>[2x]GRKKRVEISAP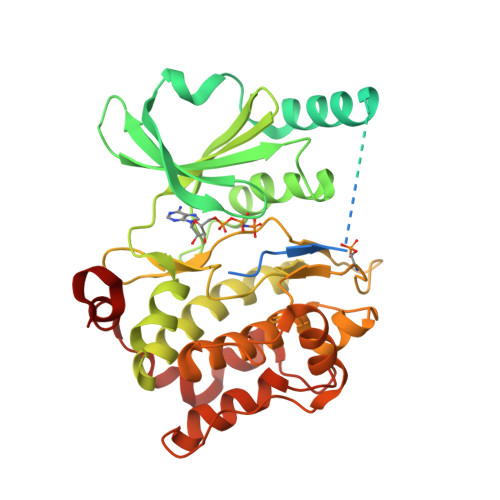SNFEHRVHTGFDQHEQKFTGLPRQWQSLIEESARRPKPLVDPACITSIQPGAPKTIVRGSKGAKDGALTLLLDEFENMSVTRSNSLRRDSPPPPARARQENGMPEKPPGPRSPQREPQRVSHEQFRAALQLVVDPGDPRSYLDNFIKIGEGSTGIVCIATVRSSGKLVAVKKMDLRKQQRRELLFNEVVIMRDYQHENVVEMYNSYLVGDELWVVMEFLEGGALTDIVTHTRMNEEQIAAVCLAVLQALSVLHAQGVIHRDIKSDSILLTHDGRVKLSDFGFCAQVSKEVPRRKSLVGTPYWMAPELISRLPYGPEVDIWSLGIMVIEMVDGEPPYFNEPPLKAMKMIRDNLPPRLKNLHKVSPSLKGFLDRLLVRDPAQRATAAELLKHPFLAKAGPPASIVPLMRQNRTR>[8x]AMAISNWVNVISDLKKIEDLIQSMHIDATLYTESDVHPSCKVTAMKCFLLELQVISLESGDASIHDTVENLIILA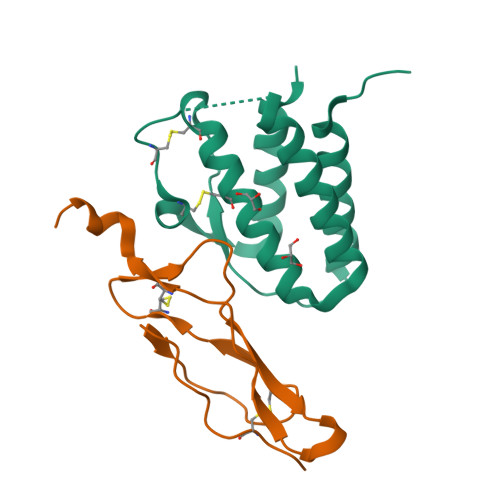NNSLSSNGNVTESGCKECEELEEKNIKEFLQSFVHIVQMFINTS;>[8x]AMAISITCPPPMSVEHADIWVKSYSLYSRERYICNSGFKRKAGTSSLTECVLNKATNVAHWTTPSLKCIRDPALVHQRPAPPSTVTTAGVTPQPESLSPSGKEPAAS> ATISFKNNCPYMVWPGTLTSDQKPQLSTTGFELASQASFQLDTPVPWNGRFWARTGCSTD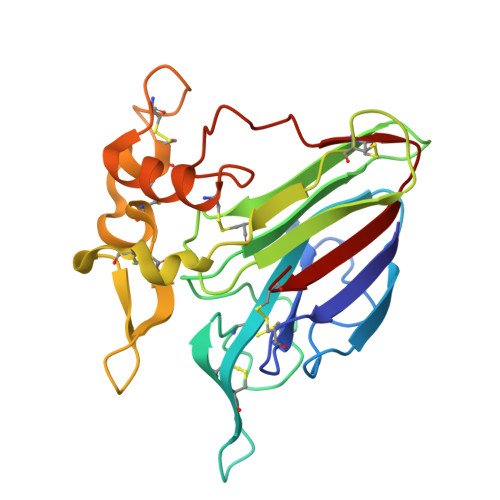ASGKFVCATADCASGQVMCNGNGAIPPATLAEFNIPAGGGQDFYDVSLVDGFNLPMSVTPQGGTGDCKTASCPANVNAVCPSELQKKGSDGSVVACLSACVKFGTPQYCCTPPQNTPETCPPTNYSEIFHNACPDAYSYAYDDKRGTFTCNGGPNYAITFCP Proper operation of the pivotal CME cargo adaptor AP2 requires membrane-localized Fer/Cip4 homology domain-only proteins (FCHO). The AP2 complex, composed of α, β2, μ2, and σ2 subunits, is pivotal to mammalian CCV formation, and its deletion is embryonically lethal in mice. FCHO1 and FCHO2 are similar in overall domain arrangement —folded N-terminal acidic phospholipid-binding homodimerization F-BAR domains and C-terminal folded μ-homology domains (μHD) separated by a ~300-residue, low-complexity intrinsically disordered protein linker, which has been suggested to participate in AP2 activation, although how it does so is undetermined. We dissect the network of interactions between the FCHO interdomain linker and AP2, which concentrates, orients, tethers, and partially destabilizes closed AP2 at the plasma membrane.

To confirm the identity of the extra, Cμ2-proximal electron density as the N terminus of FCHO2 linker, chimeras of Cμ2 alone with N1+N2 attached to the C terminus via 30-residue unstructured synthetic glycine-, serine-, and alanine-rich flexible linkers were then created, crystallized, and their structures solved at resolutions varying from 2.0 to 2.6 Å by MR using an unliganded version of Cμ2 as a search model. The Y pocket is variously filled by parts of the tags of an adjacent Cμ2 molecule. Muniscin family conserved side chains make key interactions with Cμ2 residues 167 to 170, which form the BR3 PtdIns(4,5)P2-binding site. The N1 interaction occurs mainly via complementary charged interactions between Asp318, Glu320, and Glu321 and the Cμ2 BR3 PtdIns(4,5)P2-binding site containing Lys167, Tyr168, and Arg169. Isothermal titration calorimetry (ITC) measurements showed the binding of FCHO2-N1+N2 to have a KD of ~25 μM. Mutation of key binding residues in Cμ2 (E320A+E321A+K326A) reduced binding fivefold, and mutating Tyr323 to serine rendered it unmeasurably weak. The FCHO linker does not directly interact with the Y or Ø cargo motif binding pockets in any structure but does pass close by before its main chain changes direction at FCHO2 Pro327. The weak density that follows on from N1 adopts a range of conformations forming crystal packing contacts, which we believe to be nonphysiological (mutations FCHO2 Y340S and E336A+F339S have little effect on N1-N2 binding). Whereas N1+N2 binds Cμ2 with a KD of around 25 μM, N1 alone (i.e., deletion of N2) reduces binding by ~5-fold, demonstrating that N2 plays a role in binding AP2. In support of this, mutating four of BR4’s basic residues to alanines (BR4-) caused substantial reduction in binding of GST·FCHO2 linker to Cμ2: The lower level of binding reduction of Serinc3 loop results from binding Cμ2 only at BR4 and not to BR3 (43), whereas in FCHO2, N1 can still bind to BR3 even when the BR4:N2 interaction is disrupted.

>[2x]MHHHHHHQIGWRREGIKYRRNELFLDVLESVNLLMSPQGQVLSAHVSGRVVMKSYLSGMPECKFGMNDKIVIEKQGKGTADETSKSGKQSIAIDDCTFHQCVRLSKFDSERSISFIPPDGEFELMRYRTTKDIILPFRVIPLVREVGRTKLEVKVVIKSNFKPSLLAQKIEVRIPTPLNTSGVQVICMKGKAKYKASENAIVWKIKRMAGMKESQISAEIELLPTNDKKKWARPPISMNFEVPFAPSGLKVRYLKVFEPKLNYSDHDVIKWVRYIGRSGIYETRCGASGSAGSAGPSGAGSAGSAGPSAGSAGSAGSGSAGSAPGPDVDEEGYSIKPETNQNDTKENHFYSSSDSDSEDEE>[2x]MAMETGLIFHPYMRPGRSARQTFDWGIKSAVQADSVGIDSMMISEHASQIWENIPNPELLIAAAALQTKNIKFAPMAHLLPHQHPAKLATMIGWLSQILEGRYFLGIGAGAYPQASYMHGIRNAGQSNTATGGEETKNLNDMVRESLFIMEKIWKREPFFHEGKYWDAGYPEELEGEEGDEQHKLADFSPWGGKAPEIAVTGFSYNSP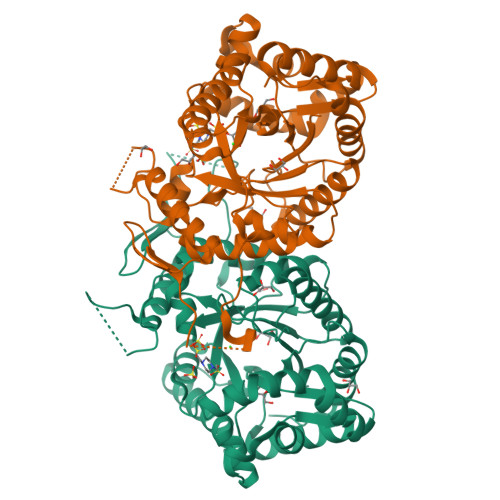SMRLAGERNFKPVSIFSGLDALKRHWEVYSEAAIEAGHTPDRSRHAVSHTVFCADTDKEAKRLVMEGPIGYCFERYLIPIWRRFGMMDGYAKDAGIDPVDADLEFLVDNVFLVGSPDTVTEKINALFEATGGWGTLQVEAHDYYDDPAPWFQSLELISKEVAPKILLPKR> QPTAPKDFSSGFWDFNDGTTQGFGVNPDSP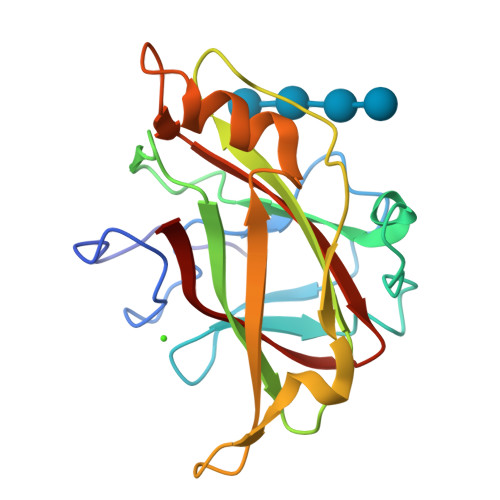ITAINVENANNALKISNLNSKGSNDLSEGNFWANVRISADIWGQSINIYGDTKLTMDVIAPTPVNVSIAAIPQSSTHGWGNPTRAIRVWTNNFVAQTDGTYKATLTISTNDSPNFNTIATDAADSVVTNMILFVGSNSDNISLDNIKFTK>[2x]MDIEERINLVLKKPTEEVLTVENLRHLFEIGAPLQHYIGFEISGYIHLGTGLMAGAKIADFQKAGIKTRVFLADWHSWINDKLGGDLEV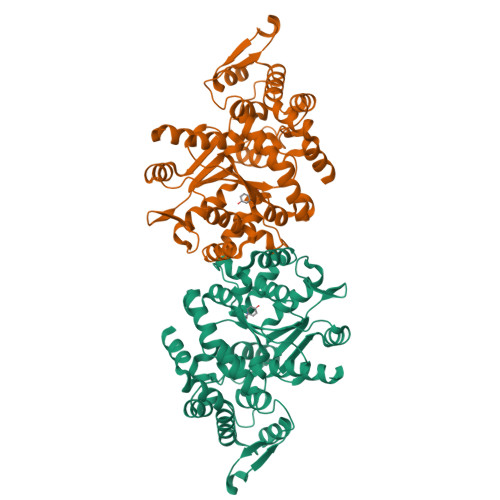IQEVALKYFKVGMEKSIEVMGGDPKKVEFVLASEILEKGDYWQTVIDISKNVTLSRVMRSITIMGRQMGEAIDFAKLIYPMMQVADIFYQGVTIAHAGMDQRKAHVIAIEVAQKLRYHPIVHEGEKLKPVAVHHHLLLGLQEPPKWPIESEEEFKEIKAQMKMSKSKPYSAVFIHDSPEEIRQKLRKAFCPAREVRYNPVLDWVEYIIFREEPTEFTVHRPAKFGGDVTYTTFEELKRDFAEGKLHPLDLKNAVAEYLINLLEPIRRYFEKHPEPLELMRSVKITR>[10x]GSASAPTLFPLVSCENSPSDTSSVAVGCLAQDFLPDSITFSWKYKNNSDISSTRGFPSVLRGGKYAATSQVLLPSKDVMQGTDEHVVCKVQHPNGNKEKNVPLPVIAELPPKVSVFVPPRDGFFGNPRKSKLICQATGFSPRQIQVSWLREGKQVGSGVTTDQVQAEAKESGPTTYKVTSTLTIKESDWLGQSMFTCRVDHRGLTFQQNASSMCVPDQDTAIRVFAIPPSFASIFLTKSTKLTCLVTDLTTYDSVTISWTRQNGEAVKTHTNISESHPNATFSAVGEASICEDDWNSGERFTCTVTHTDLPSPLKQTISRPKGVALHRPDVYLLPPAREQLNLRESATITCLVTGFSPADVFVQWMQRGQPLSPEKYVTSAPMPEPQAPGRYFAHSILTVSEEEWNTGETYTCVVAHEALPNRVTERTVDKSTGKPTLYNVSLVMSDTAGTCY;>[2x]MDSTSTIANKIEEYLGAKSDDSKIDELLKADPSEVEYYRSGGDGDYLKNNICKITVNHSDSGKYDPCEKKLPPYDDNDQWKCQQNSSDGSGKPENICVPPRRERLCTYNLENLKFDKIRDNNAFLADVLLTARNEGEKIVQNHPDTNSSNVCNALERSFADLADIIRGTDQWKGTNSNLEKNLKQMFAKIRENDKVLQDKYPKDQKYTKLREAWWNANRQKVWEVITCGARSNDLLIKRGWRTSGKSDRKKNFELCRKCGHYEKEVPTKLDYVPQFLRWLTEWIEDFYREKQNLIDDMERHREECTREDHKSKEGTSYCSTCKDKCKKYCECVKKWKTEWENQENKYKDLYEQNKNKTSQKNTSRYDDYVKDFFEKLEANYSSLENYIKGDPYFAEYATKLSFILNPSDANNPSGETANHNDEACNCNESGISSVGQAQTSGPSSNKTCITHSSIKTNKKKECKDVKLGVRENDKDLKICVIEDTSLSGVDNCCCQDLLGILQENCSDNKRGSSSNDSCDNKNQDECQKKLEKVFASLTNGYKCDKCKSGTSRSKKKWIWKKSSGNEEGLQEEYANTIGLPPRTQSLYLGNLPKLENVCEDVKDINFDTKEKFLAGCLIVSFHEGKNLKKRYPQNKNSGNKENLCKALEYSFADYGDLIKGTSIWDNEYTKDLELNLQNNFGKLFGKYIKKNNTAEQDTSYSSLDELRESWWNTNKKYIWTAMKHGAEMNITTCNADGSVTGSGSSCDDIPTIDLIPQYLRFLQEWVENFCEQRQAKVKDVITNCKSCKESGNKCKTECKTKCKDECEKYKKFIEACGTAGGGIGTAGSPWSKRWDQIYKRYSKHIEDAKRNRKAGTKNCGTSSTTNAAASTDENKCVQSDIDSFFKHLIDIGLTTPSSYLSNVLDDNICGADKAPWTTYTTYTTTEKCNKERDKSKSQSSDTLVVVNVPSPLGNTPYRYKYACQCKIPTNEETCDDRKEYMNQWSCGSARTMKRGYKNDNYELCKYNGVDVKPTTVRSNSSKLDGNDVTFFNLFEQWNKEIQYQIEQYMTNANISCIDEKEVLDSVSDEGTPKVRGGYEDGRNNNTDQGTNCKEKCKCYKLWIEKINDQWGKQKDNYNKFRSKQIYDANKGSQNKKVVSLSNFLFFSCWEEYIQKYFNGDWSKIKNIGSDTFEFLIKKCGNNSAHGEEIFSE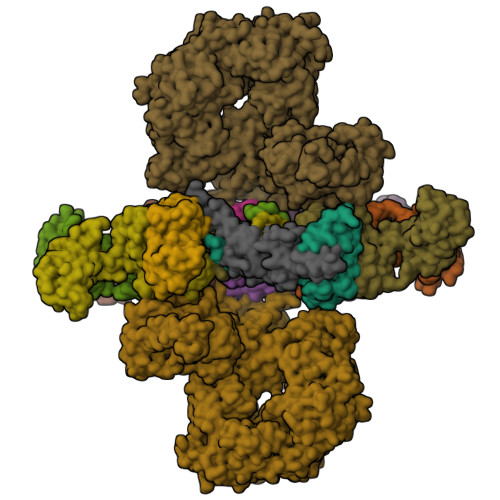KLKNAEKKCKENESTDTNINKSETSCDLNATNYIRGCQSKTYDGKIFPGKGGEKQWICKDTIIHGDTNGACIPPRTQNLCVGELWDKSYGGRSNIKNDTKELLKEKIKNAIHKETELLYEYHDTGTAIISKNDKKGQKGKNDPNGLPKGFCHAVQRSFIDYKNMILGTSVNIYEHIGKLQEDIKKIIEKGTPQQKDKIGGVGSSTENVNAWWKGIEREMWDAVRCAITKINKKNNNSIFNGDECGVSPPTGNDEDQSVSWFKEWGEQFCIERLRYEQNIREACTINGKNEKKCINSKSGQGDKIQGACKRKCEKYKKYISEKKQEWDKQKTKYENKYVGKSASDLLKENYPECISANFDFIFNDNIEYKTYYPYGDYSSICSCEQVKYYKYNNAEKKNNKSLCYEKDNDMTWSKKYIKKLENGRSLEGVYVPPRRQQLCLYELFPIIIKNEEGMEKAKEELLETLQIVAEREAYYLWKQYNPTGKGIDDANKKACCAIRGSFYDLEDIIKGNDLVHDEYTKYIDSKLNEIFGSSNTNDIDTKRARTDWWENETITNGTDRKTIRQLVWDAMQSGVRYAVEEKNENFPLCMGVEHIGIAKPQFIRWLEEWTNEFCEKYTKYFEDMKSKCDPPKRADTCGDNSNIECKKACANYTNWLNPKRIEWNGMSNYYNKIYRKSNKESEDGKDYSMIMAPTVIDYLNKRCHGEINGNYICCSCKNIGAYNTTSGTVNKKLQKKETECEEEKGPLDLMNEVLNKMDKKYSAHKMKCTEVYLEHVEEQLNEIDNAIKDYKLYPLDRCFDDQTKMKVCDLIADAIGCKDKTKLDELDEWNDMDLRGTYNKHKGVLIPPRRRQLCFSRIVRGPANLRSLNEFKEEILKGAQSEGKFLGNYYKEHKDKEKALEAMKNSFYDYEDIIKGTDMLTNIEFKDIKIKLDRLLEKETNNTKKAEDWWKTNKKSIWNAMLCGYKKSGNKIIDPSWCTIPTTETPPQFLRWIKEWGTNVCIQKQEHKEYVKSKCSNVTNLGAQASESNNCTSEIKKYQEWSRKRSIQWETISKRYKKYKRMDILKDVKEPDANTYLREHCSKCPCGFNDMEEMNNNEDNEKEAFKQIKEQVKIPAELEDVIYRIKHHEYDKGNDYICNKYKNIHDRMKKNNGNFVTDNFVKKSWEISNGVLIPPRRKNLFLYIDPSKICEYKKDPKLFKDFIYWSAFTEVERLKKAYGGARAKVVHAMKYSFTDIGSIIKGDDMMEKNSSDKIGKILGDTDGQNEKRKKWWDMNKYHIWESMLCGYREAEGDTETNENCRFPDIESVPQFLRWFQEWSENFCDRRQKLYDKLNSECISAECTNGSVDNSKCTHACVNYKNYILTKKTEYEIQTNKYDNEFKNKNSNDKDAPDYLKEKCNDNKCECLNKHIDDKNKTWKNPYETLEDTFKSKCDCPKPLPSPIKPDDLPPQADEPFLESRGPFEGKPIPNPLLGLDSTRTGHHHHHH;> EDERIVLVDNKCKCARITSRIIRSSEDPNEDIVERNIRIIVPLNNRENISDPTSPLRTRFVYHLSDLCKKCDPTEVELDNQIVTATQSNICDEDSATETCYTYDRNKCYTAVVPLVYGGETKMVETALTPDACYPD> GLAHSSCSPGGDPTAGAAWACFRLDGRTLLRVRGPDAAPFLLGLLTNELPLPSPAAAGAPPAARAGYAHFLNVQ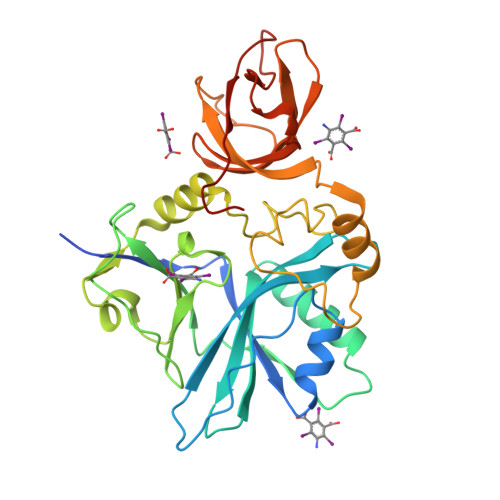GRTLYDVILYGLQEHSEVSGFLLECDSSVQGALQKHLALYRIRRKVTVEPHPELRVWAVLPSSPEACGAASLQERAGAAAILIRDPRTARMGWRLLTQDEGPALVPGGRLGDLWDYHQHRYLQGVPEGVRDLPPGVALPLESNLAFMNGVSFTKGCYIGQELTARTHHMGVIRKRLFPVRFLDPLPTSGITPGATVLTASGQTVGKFRAGQGNVGLALLWSEKIKGPLHIRASEGAQVALAASVPDWWPTVSK>MCTRAVYLGPDRMVVTGRTMDWKEDIMSNIYVFPRGMQRAGHNKEKTVNWTSKYGSVIATGYDIGTCDGMNEKGLVASLLFLPESVYSLPGDTRPAMGISIWTQYVLDNFATVREAVDEMKKETFRIDAPRMPNGGPESTLHMAITDETGNTAVIEYLDGKLSIHEGKEYQVMTNSPRYELQLAVNDYWKEVGGLQMLPGTNRSSDRFVRASFYIHAIPQTADAKIAVPSVLSVMRNVSVPFGINTPEKPHISSTRWRSVSDQKNKVYYFESTLTPNLFWLDLKKIDFSPKAGVKKLSLTKGEIYAGDAVKDLKDSQSFTFL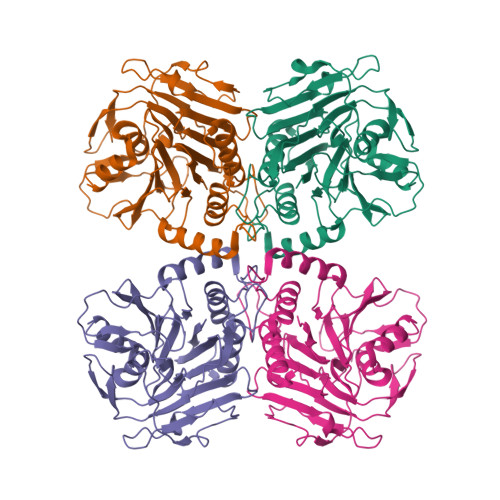FETPVMLEHHHHHH[4x]> QSVTQPDARVTVSEGASLQLRCKYSYSA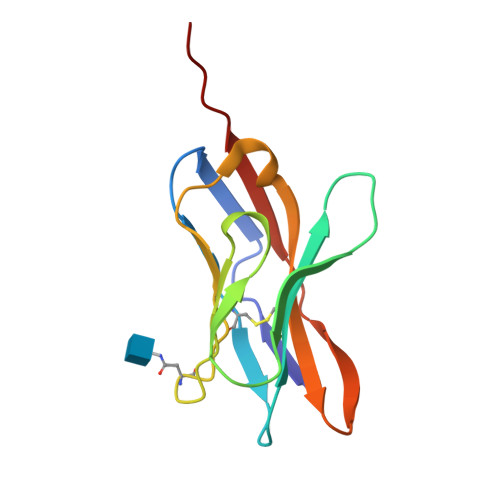TPYLFWYVQYPRQGLQLLLKYYSGDPVVQGVNGFEAEFSKSNSSFHLRKASVHWSDSAVYFCAVSGFASALTFGSGTKVIVLPYIQN> YDPDQYSIEADKKFKYSVKLSDYPTLQDAASAAVDGLLIDRDYNFYGGETVDFGGKVLTIECKAKFIGDGNLIFTKLGKGSRIAGVFMESTTTPWVIKPWTDDNQWLTDAAAVVATLKQSKTDGYQPTVSDYVKFPGIETLLPPNAKGQNITSTLEIRECIGVEVHRASGLMAGFLFRGCHFCKMVDA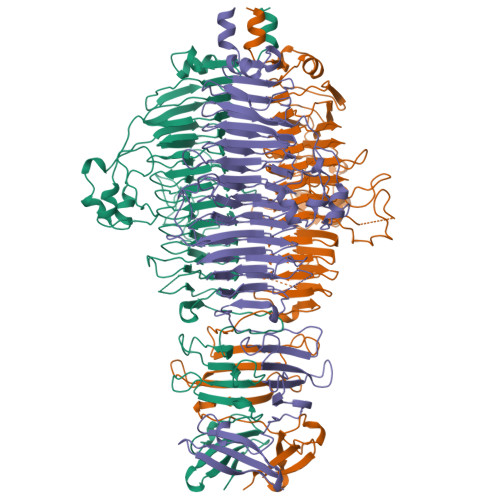NNPSGGKDGIITFENLSGDWGKGNYVIGGRFSYGSVSSAQFLRNNGGFERDGGVIGFTSYRAGESGVKTWQGTVGSTTSRNYNLQFRDSVVIYPVWDGFDLGADTDMNPELDRPGDYPITQYPLHQLPLNHLIDNLLVRGALGVGFGMDGKGMYVSNITVEDCAGSGAYLLTHESVFTNIAIIDTNTKDFQANQIYISGACRVNGLRLIGIRSTDGQSLTIDAPNSTVSGITGMVDPSRINVANLAEEGLGNIRANSFGYDSAAIKLRIHKLSKTLDSGALYSHINGGAGSGSAYTQLTAISGSTPDAVSLKVNHKDCRGAEIPFVPDIASDDFIKDSSCFLPYWENNSTSLKALVKKPNGELVRLTLATL>[2x]PDIFNRDPRDHYD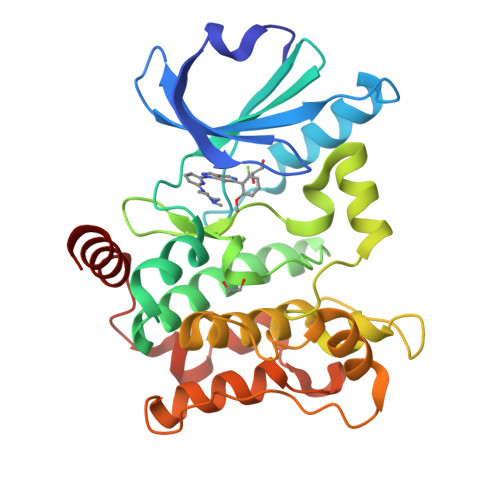LLQRLGGGTYGEVFKARDKVSGDLVALKMVKMEPDDDVSTLQKEILILKTCRHANIVAYHGSYLWLQKLWICMEFCGAGSLQDIYQVTGSLSELQISYVCREVLQGLAYLHSQKKIHRDIKGANILINDAGEVRLADFGISAQIGATLARRLAFIGTPYWMAPEVAAVALKGCYNELCDIWSLGITAIELAELQPPLFDVHPLRVLFLMTKSGYQPPRLKEKGKWSAAFHNFIKVTLTKSPKKRPSATKMLSHQLVSQPGLNRGLILDLLDKLKNP> GSHMASMFGKLREKLKSFVKRVEEEVEKEEEEVEKKGLLDRILTVEIKEKDVDKALDELEIDLLEADVALEVVDALREKIKQKLVGKKVRIGTDKGKIIEEAVKEAVSEILETSRRIDLIEEIRKAEKPYVIMFVGFNGSGKTTTIAKLANWLKNHGFSVVIAASDTFRAGAIEQLEEHA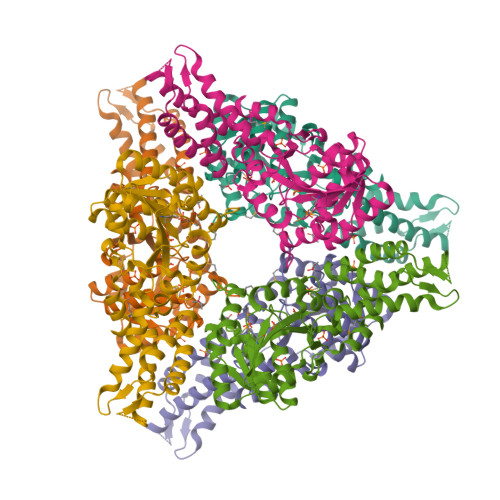KRIGVKVIKHSYGADPAAVAYDAIQHAKARGIDVVLIDTAGRSETNRNLMDEMKKIARVTKPNLVIFVGDALAGNAIVEQARQFNEAVKIDGIILTKLDADARGGAALSISYVIDAPILFVGVGQGYDDLRPFEKEWFLERIFGEENA>AACCCC[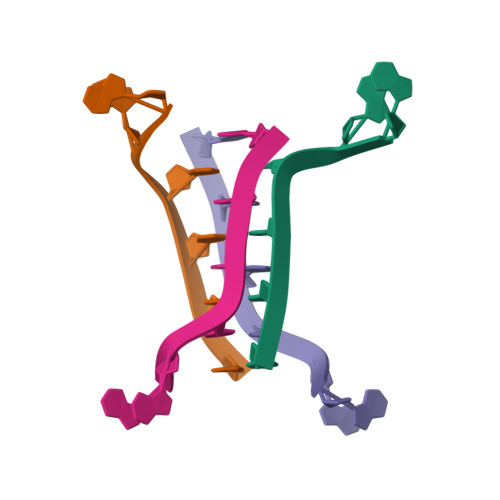8x]> DLKWHHHNITYWIQNYSEDLPRAVID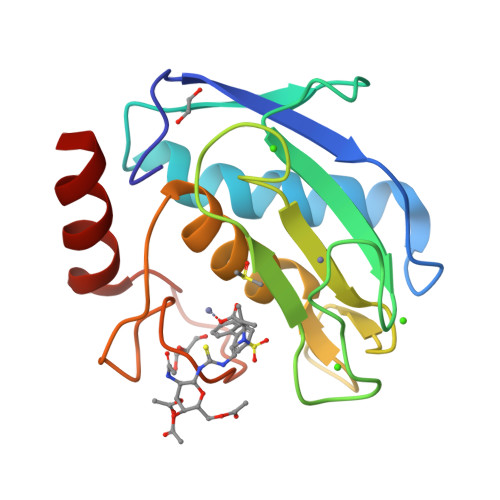DAFARAFALWSAVTPLTFTRVYSRDADIVIQFGVAEHGDGYPFDGKDGLLAHAFPPGPGIQGDAHFDDDELWSLGKGVGYSLFLVAAHEFGHALGLDHSSVPEALMYPMYRFTEGPPLHKDDVNGIRHLYG>[2x]MTKVFAYAIRKDEEPFLNEWKEAHKDIDVDYTDKLLTPETAKLAKGADGVVVYQQLDYTADTLQALADAGVTKMSLRNVGVDNIDMDKAKELGFQITNVPVYSPNAIAEHAAIQAARVLRQDKRMDEKMAKRDLRWAPTIGREVRDQVVGVVGTGHIGQVFMRIM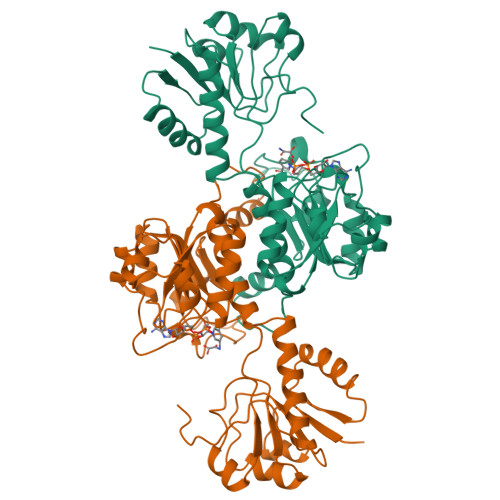EGFGAKVIAYDIFKNPELEKKGYYVDSLDDLYKQADVISLHVPDVPANVHMINDKSIAEMKDGVVIVNCSRGRLVDTDAVIRGLDSGKIFGFVMDTYEDEVGVFNKDWEGKEFPDKRLADLIDRPNVLVTPHTAFYTTHAVRNMVVKAFNNNLKLINGEKPDSPVALNKNKF>MRIGYGEDSHRLEEGRPLYLCGLLIPSPVGALAHSDGDAAMHALTDALLSAYGLGDIGLLFPDTDPRWRGERSEVFLREAMRLVEARGAKLLQASLVLTLDRPKLGPHRKALVDSLSRLMRLPQDRIGLTFKTSEGLA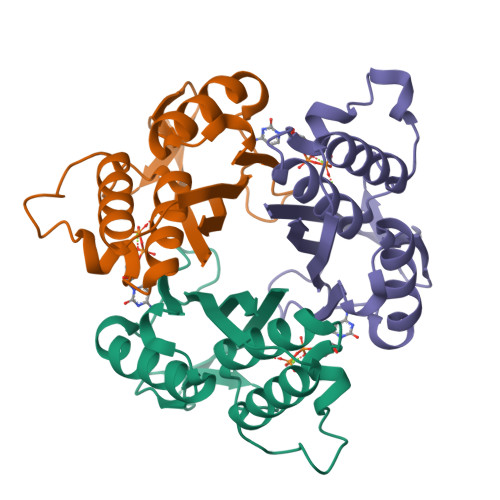PSHVQARAVVLLDG[6x]>[3x]VDISTLPRVKVDLVKPPFVHAHDQVAKTGPRVVEFTMTIEEKKLVIDREGTEIHAMTFNGSVPGPLMVVHENDYVELRLINPDTNTLLHNIDFHAAT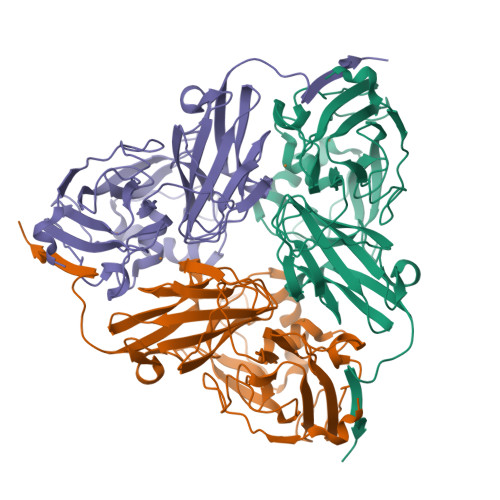GALGGGALTQVNPGEETTLRFKATKPGVFVYHCAPEGMVPWHVTSGMNGAIMVLPRDGLKDEKGQPLTYDKIYYVGEQDFYVPKDEAGNYKKYETPGEAYEDAVKAMRTLTPTHIVFNGAVGALTGDHALTAAVGERVLVVHSQANRDTRPHLIGGHGDYVWATGKFRNPPDLDQETWLIPGGTAGAAFYTFRQPGVYAYVNHNLIEAFELGAAGHFKVTGEWNDDLMTSVVKPASM>MGGSFGKKGASSATAAQVPLATETTPGLMSP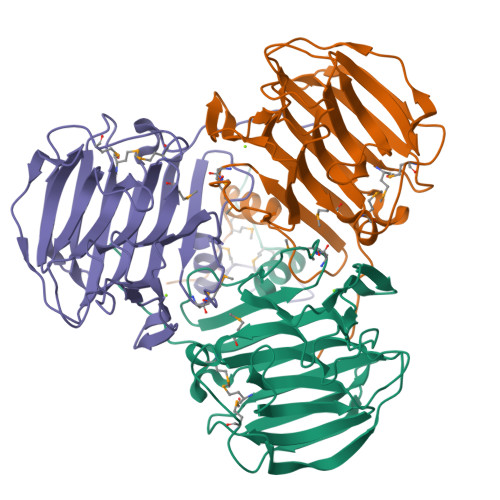SEKLKLSTLTTSIATSDFYASYDFMMHSIGLTSANNISLLSTGNISLQNILSEGNHFGVQPIVSSTTANASFLAGMLMAIFPKESELEVTVYFKTPSAFNPAQLTVIGSTSIGLGISDRSGLIIENGNAFGGIVKASAATETGSTYALSTSTWYICKFKMLTDDRFKVTLYSDSGTQLYSYTSTAAMFRADNATAHIGFKTQCKTATAGISLISIDLIEFKAKVSATRAKV[3x]>[2x]FDIDMVFSWVDGSDPEFRARRMAQMSQY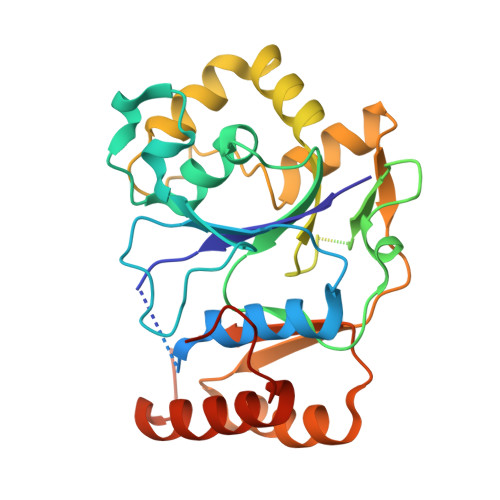VVGEGDDAEARIRQIDELKYALRSVNMFAPWIRRIFIATDSTPPPWLAEHPKITIVRAEDHFSDRSALPTYNSHAVESQLHHIPGLSEHFLYSNDDMFFGRPLKASMFFSPGGVTRFIEAKTRIGLGANNPARSGFENAARVNRQLLFDRFGQVITRHLEHTAVPLRKSVLIEMEREFPEEFARTAASPFRSDTDISVTNSFYHYYALMTGRAVPQEKAKVLYVDTTSYAGLRLLPKLRKHRGYDFFCLNDGSFPEVPAAQRAERVVSFLERYFPIPAPWEKIAADVSRRDF>AGGKVTSSTGIAPKRYVYYPGSEELGPDEIRVIACGTGMPTARRAQAAAAWVVELGNGDKFIVDIGSGSMANIQSLMIPANYLTKIFLTHLHTDHWGDLVSMWAGGWTAGRTDPLEVWGPSGSREDMGTKYAVEHMLKAYNWDYMTRAVTINPRPGDINVHEFDYRALNEV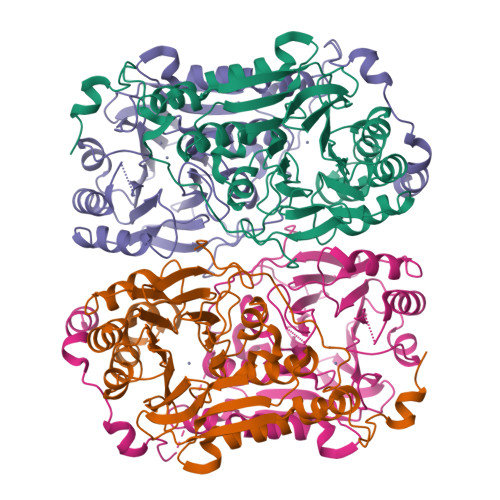VYQENGVTFRSWPCIHAGDGPVSFALEWNGYKVVFGGDTAPNIWYPEYAKGADLAIHECWMTSDQMMTKYNQPAQLALRINLDFATSAQSFGQIMNMVQPRHAVAYHFFNDDDTRYDIYTGVRENYAGPLSMATDMMVWNITRDAVTERMAVSPDHAWDVAGPSEDLAPDRNRASEYTQYILDGRLNVDEANAHWKQEFMG[4x]[3-(4-{2-[3,5-difluoro-4-(1-methyl-1,2,3,6-tetrahydropyridin-4-yl)anilino]-7H-pyrrolo[2,3-d]pyrimidin-4-yl}-1H-pyrazol-1-yl)-1-(ethanesulfonyl)azetidin-3-yl]acetonitrile | C28 H29 F2 N9 O2 S | 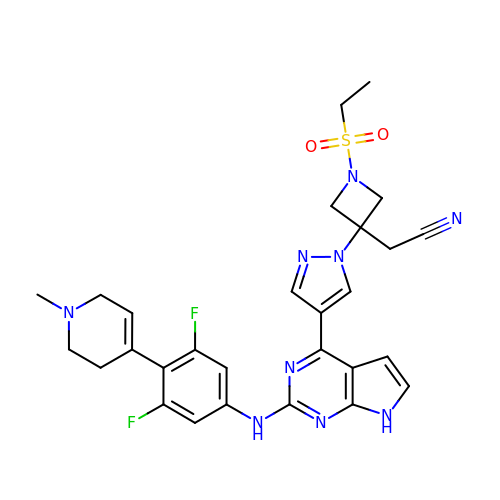MXGPFEUZRMBECL-UHFFFAOYSA-N(3R,4S)-1-[(4-amino-5H-pyrrolo[3,2-d]pyrimidin-7-yl)methyl]-4-(2-{[2-(2-hydroxyethoxy)ethyl]sulfanyl}ethyl)pyrrolidin-3-ol | 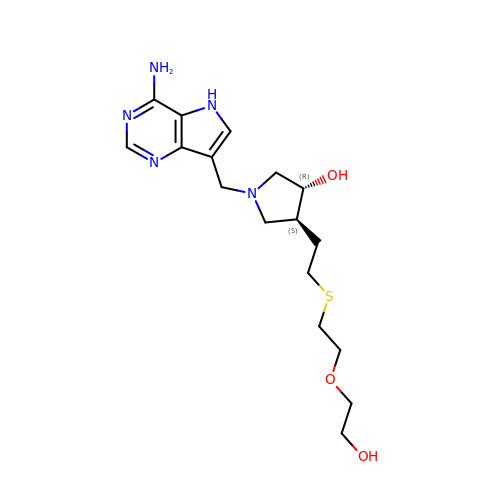C17 H27 N5 O3 S | NLPFBCRTOQVKFZ-JSGCOSHPSA-N>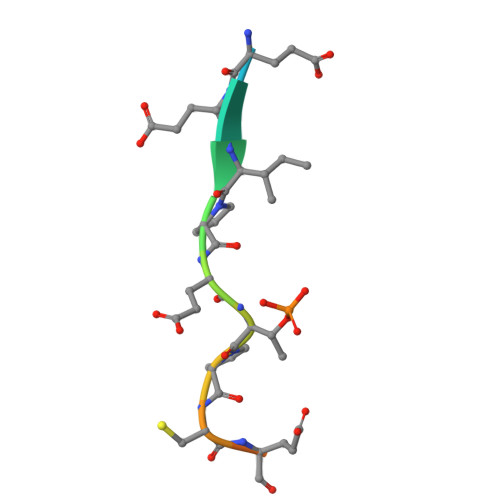 EVEEIPETPCESQGE>[4x]GPGSMTDITYRLAQKRTIVTPLPGPRSGALAERRRAAVSAGVGSTAPVYAVDADGGVIVDADGNSFIDLGAGIAVTTVGASHPAVAAAIADQATHFTHTCFMVTPYEQYVQVAELLNALTPGDHDKRTALFNSGAEAVENAIKVARLATGRPAVVAFDNAYHGRTNLTMALTAKSMPYKSQFGPFAPEVYRMPAS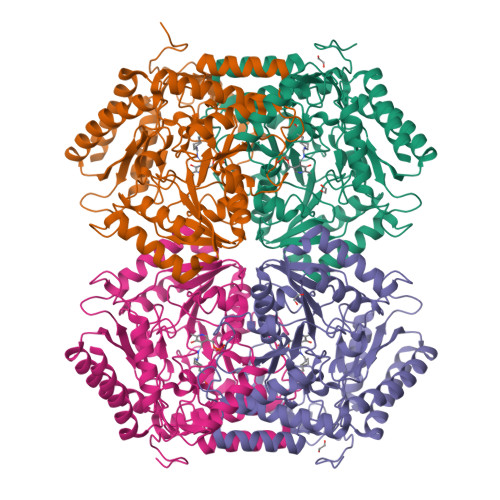YPLRDEPGLTGEEAARRAISRIETQIGAQSLAAIIIEPIQGEGGFIVPAPGFLATLTAWASENGVVFIADEVQTGFARTGAWFASEHEGIVPDIVTMAKGIAGGMPLSAVTGRAELMDAVYAGGLGGTYGGNPVTCAAAVAALGVMRELDLPARARAIEASVTSRLSALAEEVDIIGEVRGRGAMLAIEIVKPGTLEPDAALTKSIAAEALSQGVLILTCGTFGNVIRLLPPLVIGDDLLDEGITALSDIIRAKASHQ>[3x]MAHHHHHHMNLRAAGPGWLFCPADRPERFAKAAAAADVVILDLEDGVAEAQKPAARNALRDTPLDPERTVVRINAGGTADQARDLEALAGTAYTTVMLPKAESAAQVIELAPRDVIALVETARGAVCAAEIAAADPTVGMMWGAEDLIATLGGSSSRRADGAYRDVARHVRSTILLAASAFGRLALDAVHLDILDVEGLQEEARDAAAVGFDVTVCIHPSQIPVVRKAYRPSHEKLAWARRVLAASRSERGAFAFEGQMVDSPVLTHAETMLRRAGEATSE

Mtb protein Rv2498c is currently annotated as the β-subunit (CitE) of the heterotrimeric prokaryotic citrate lyase complex involved in TCA cycle cataplerosis. Combining phylogenetic analysis, in vitro enzymatic assays, in vivo Mtb experiments, and X-ray crystallography, we identified Mtb Rv2498c as an essential stereospecific bifunctional β-hydroxyacyl-CoA lyase (β-HAC lyase) that carries out the last step of itaconate dissimilation pathway and confers resistance to itaconate. A systematic evaluation of substrate specificity revealed (R)-HMG-CoA ∼ (S)-citramalyl-CoA >>> (S)-malyl-CoA ∼ β-methylmalyl-CoA as substrates for Rv2498c. To investigate the molecular basis of Rv2498c substrate stereospecificity for the carbon–carbon bond, we determined the structures of Rv2498c in a variety of liganded states by X-ray crystallography.

In contrast to the previously reported structures, the C terminus (50 residues) is well ordered in our structures, forming an α-helix/β-hairpin/α-helix motif that packs against the surface of the neighboring protomer, capping its active site. The fact that the C terminus is ordered in these ligand-bound structures is consistent with earlier observations that the position and organization of the C terminus might depend on the occupancy of the active site. The CoA moiety binds in a deep cleft at the base of which resides the active site Mg2+ ion. Rv2498c catalyzed the carbon–carbon bond cleavage of (S)-citramalyl-CoA to form pyruvate and Ac-CoA (kcat/Km = 2.3 × 105). Itaconate dissimilation in Mtb involves the bifunctional enzyme Rv2498c, which cleaves (S)-citramalyl-CoA producing Ac-CoA and pyruvate, effectively using a host-derived antibacterial molecule as a nutrient source.> KKQCGVLEGLKVKSEWGRAYGSGHDREAFSQAIWRATFAQVPESRSLFKRVHGDDTSHPAFIAHADRVLGGL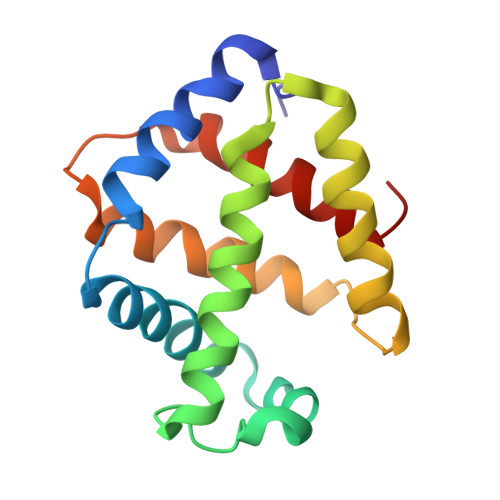DIAISTLDQPATLKEELDHLQVQHEGRKIPDNYFDAFKTAILHVVAAQLGRCYDREAWDACIDHIEDGIKGHH(4R)-4-hydroxy-D-proline | C5 H9 N O3 | 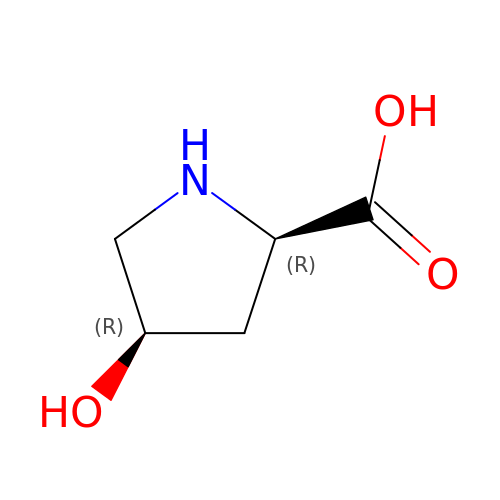PMMYEEVYMWASQN-QWWZWVQMSA-N> MKVGQDKVVTIRYTLQVEGEVLDQGELSYLHGHRNLIPGLEEALEGREEGEAFQAHVPAEKAYGPHDPEGVQVVP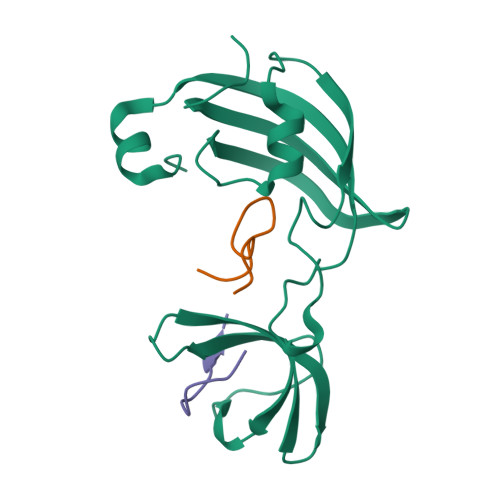LSAFPEDAEVVPGAQFYAQDMEGNPMPLTVVAVEGEEVTVDFNHPLAGKDLDFQVEVVKVREATPEELLHGHAHPGHHHHHH;>TRYKNAKMLPFAFGA[2x]Cleavage and polyadenylation factor (CPF/CPSF) is a multi-protein complex essential for formation of eukaryotic mRNA 3ʹ ends. CPF cleaves pre-mRNAs at a specific site and adds a poly(A) tail. In contrast, there is little mechanistic information available on the nuclease module, which is composed of the endonuclease Ysh1/CPSF73, the pseudo-nuclease Cft2/CPSF100, and the multi-domain protein Mpe1/RBBP6 (Casañal et al., 2017). In vivo studies and reconstitution assays using extracts found that many of the CPF subunits were required for nuclease activity (Zhao et al., 1999) and that Ysh1/CPSF73 is the enzymatic component (Chanfreau et al., 1996, Dominski, 2010, Jenny et al., 1996, Ryan et al., 2004).

To investigate the molecular details of the Ysh1-Mpe1 interaction, we determined the X-ray crystal structure of a complex between the catalytic domain of Ysh1 (residues 1–473) and the UBL domain of Mpe1 (residues 1–120). The structure was refined to 2.3 Å resolution. Ysh1 adopts a globular fold comprised of a metallo-β-lactamase and β-CASP domain, similar to the human 3ʹ endonuclease CPSF73 and yeast Cft2 (Mandel et al., 2006). Residues H68, H70, D72, H73, H163, D184, and H430 comprise the active site, coordinating two Zn2+ ions with octahedral geometry. The catalytic core is located in a large internal solvent-filled cavity at the boundary between the metallo-β-lactamase and β-CASP domains, with a narrow tunnel leading to the surface of the enzyme. The UBL domain of Mpe1 consists of a central α helix flanked by a curved 4-stranded β sheet and capped by an additional pair of short anti-parallel β strands, in the same configuration as the UBL domain of the human ortholog RBBP6 (root mean square deviation [RMSD] = 1.36 Å over 452 atoms; (Pugh et al., 2006)). The interface between Mpe1 and Ysh1 buries an area of ∼900 Å2 and involves hydrophobic, polar, and electrostatic contacts between Mpe1 residues in loops and β strands and Ysh1 residues on the top surface of the metallo-β-lactamase domain. Mpe1 binds to the Ysh1 metallo-β-lactamase domain next to the active site tunnel opening. A large basic patch is formed by contiguous surfaces of both Ysh1 and Mpe1, suggesting a possible role in RNA binding. However, in the structure, Ysh1 remains in a “closed” conformation that is unlikely to be catalytically active because the active site tunnel is too narrow to accommodate the entire RNA substrate.

> MERTNTTTFKFFSLGGSNEVGRSCHILQYKGKTVMLDAGIHPAYQGLASLPFYDEFDLSKVDILLISHFHLDHAASLPYVMQRTNFQGRVFMTHPTKAIYRWLLRDFVRVTSIGSSSSSMGTKDEGLFSDEDLVDSFDKIETVDYHSTVDVNGIKFTAFHAGHVLGAAMFQIEIAGLRVLFTGDYSREVDRHLNSAEVPPLSSNVLIVESTFGTATHEPRLNRERKLTQLIHSTVMRGGRVLLPVFALGRAQEIMLILDEYWSQHADELGGGQVPIFYASNLAKKCMSVFQTYVNMMNDDIRKKFRDSQTNPFIFKNISYLRNLEDFQDFGPSVMLASPGMLQSGLSRDLLERWCPEDKNLVLITGYSIEGTMAKFIMLEPDTIPSINNPEITIPRRCQVEEISFAAHVDFQENLEFIEKISAPNIILVHGEANPMGRLKSALLSNFASLKGTDNEVHVFNPRNCVEVDLEFQG;> MSSTIFYRFKSQRNTSRILFDGTGLTVFDLKREIIQENKLGDGTDFQLKIYNPDTEEEYDDDAFVIPRSTSVIVKRSPAIKSFSVHSRLKGNVGAAAKGNATRYVTGRPRVLQKRQHTATTTANVSGTTEEERIASMFATQENQWEQTQEEMSAATPVFF> PRQWQSLIEESARRPKPLVD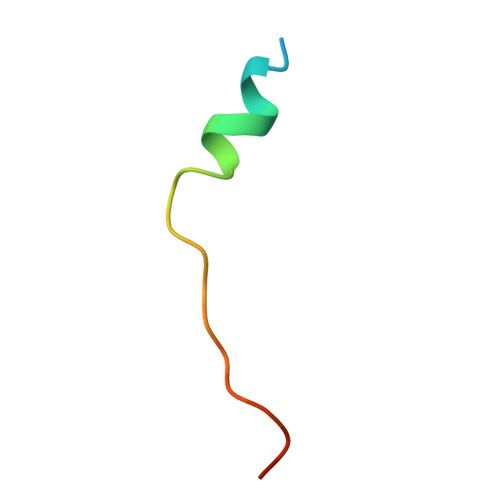PACIT>[4x]MRIPLVGKDSIESKDIGFTLIHEH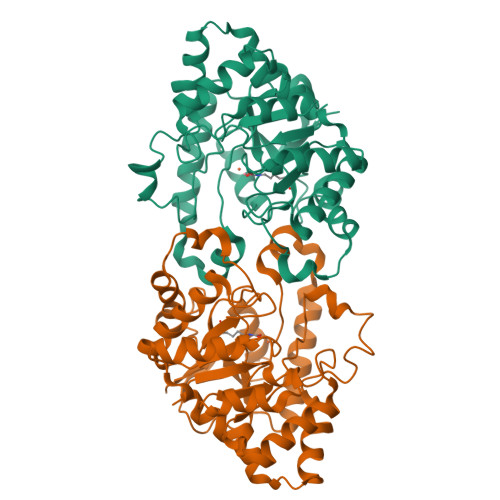LRVFSEAVRQQWPHLYNEDEEFRNAVNEVKRAMQFGVKTIVDPTVMGLGRDIRFMEKVVKATGINLVAGTGIYIYIDLPFYFLNRSIDEIADLFIHDIKEGIQGTLNKAGFVKIAADEPGITKDVEKVIRAAAIANKETKVPIITHSNAHNNTGLEQQRILTEEGVDPGKILIGHLGDTDNIDYIKKIADKGSFIGLDRYGLDLFLPVDKRNETTLRLIKDGYSDKIMISHDYCCTIDLGTAKPEYKPKLAPRWSITLIFEDTIPFLKRNGVNEEVIATIFKENPKKFFS> GGLEKDFLPLYFGWFLTKKSSETLRKAGQVFLEELGNHKAFKKELRHFISGDEPKEKLELVSYFGKRPPGVLHCTTKFCDYGKAAGAEEY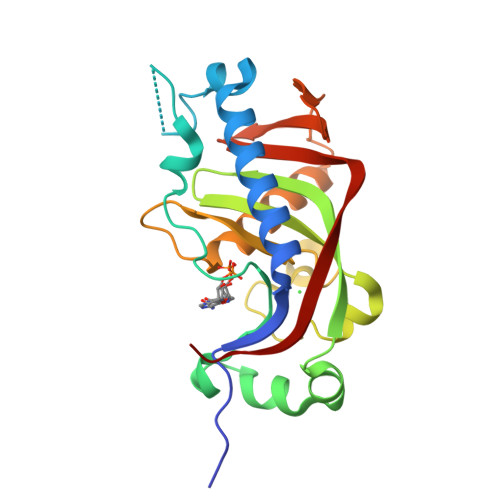AQQEVVKRSYGKAFKLSISALFVTPKTAGAQVVLTDQELQLWPSDLDKPSASEGLPPGSQAHVTLGCAADVQPVQTGLDLLDILQQVKGGSQGEAVGELPRGKLYSLGKGRWMLSLTKKMEVKAIFTGYYG>SDAKRIEGFTLSEEILKSDKQLSVDAQFFTKPLTDGMAIRSEGKIYFVDKQASLSDGLWLVDIEGAISIRELTKLPGRKLHV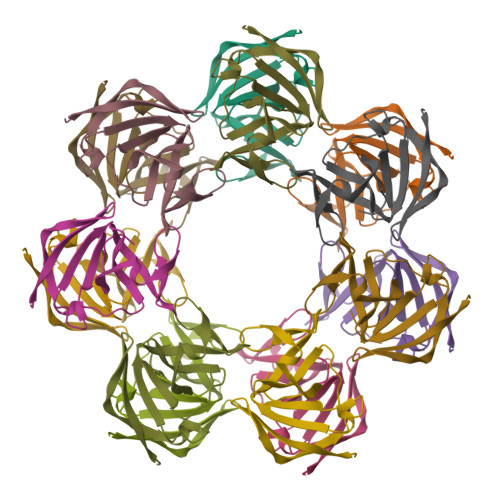AGGKVPFECGIDDIKTLGRVVGVYSEVN[14x]> S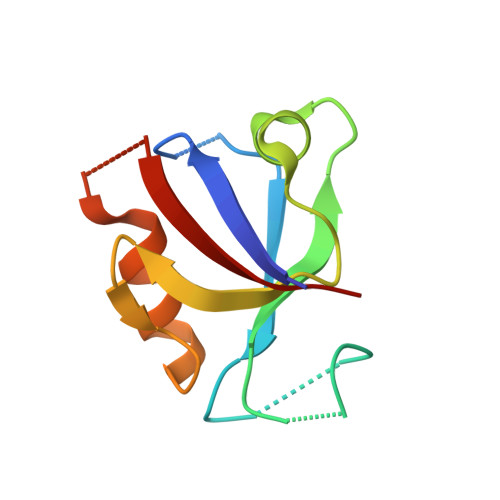VEEIRLPRAGGPLGLSIVGGSDHSSHPFGVQEPGVFISKVLPRGLAARSGLRVGDRILAVNGQDVRDATHQEAVSALLRPCLELSLLVRRD>GSHMGGIEVLDVKTGPDSTTTIEAYLNPRVGQNWGFSTEITVASNGYNDAPHLTEIPCYSSARISLPLLNEDITSPTLLMWEAVSVKTEVVGISSMLNMHSYGLRAFGGYGGGYTIEGSHIHFFSVGGEPLDLQGLMQNHSTQYPSPLVGPKKPDGTTDDSAQVLNPIYKAKLDKDATYPIECWCPDPSRNENSRYFGSYTGGVETPPVLSFTNTSTTILLDENGVGPLCKGDGLYLSSA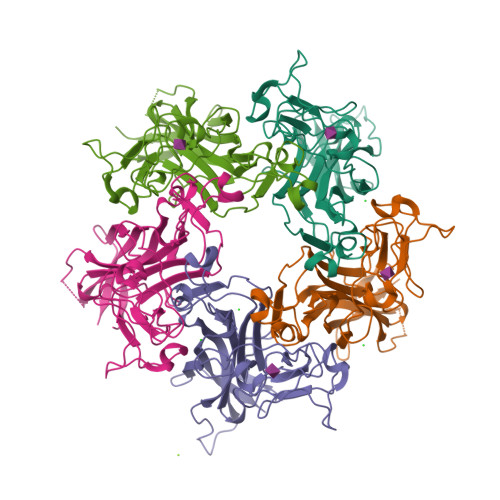DVAGTFVQQTSQKQYWRGLPRYFNITLRKRAVKN[40x]3-[1-[2-(4-METHYLPHENOXY)ETHYL]BENZIMIDAZOL-2-YL]SULFANYLPROPANOIC ACID | C19 H20 N2 O3 S | 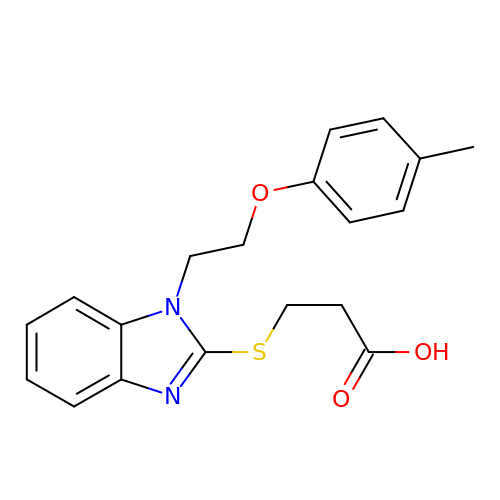KGCGDYADLNUQIH-UHFFFAOYSA-N> MTESYDVVVVGGGPVGLATAWQVAERGHRVLVLERHTFFNENGGTSGAERHWRLQYTQEDLFRLTLETLPLWRALESRCERRLIHEIGSLWFGDTDVVTNEGQISGTAAMMDKLSVRYEWLKATDIERRFGFRGLPRDYEGFLQPDGGTIDVRGTLAALFTLAQAAGATLRAGETVTELVPDADGVSVTTDRGTYRAGKVVLACGPYTNDLLEPLGARLAYSVYEMAIAAYRQATP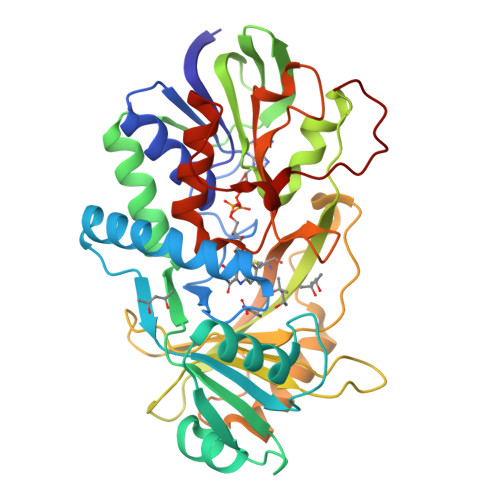VTEAPFWFAFQQPTPQDTNLFFGFGHNPWAPGEFVRCGPDFEVDPLDHPSAATGVADRRQMDRLSGWLRDHLPTVDPDPVRTSTCLAVLPTDPERQFFLGTARDLMTHGEKLVVYGAGWAFKFVPLFGRICADLAVEDSTAYDISRLAPQSALLEHHHHHH> MSLRIDVDTNFPECVVDAGKVTLGTQQRQEMDPRLREKQNEIILRAVCALLNSGGGIIKAEIENKGYNYERHGVGLDVPPIFRSHLDKMQKENHFLIFVKSWNTEAGVPLATLCSNLYHRERTSTDVMDSQEALAFLKCRTQTPTNINVSNSLGPQAAQGSVQYEGNINVSAAALFDRKRLQYLEKLNLPESTHVEFVMFSTDVSHCVKDRLPKCVSAFANTEGGYVFFGVHDETCQVIGCEKEKIDLTSLRASIDGCIKKLPVHHFCTQRPEIKYVLNFLEVHDKGALRGYVCAIKVEKFCCAVFAKVPSSWQVKDNRVRQLPTREWTAWMMEADLEHHHHHH

The Schlafen family belongs to the interferon-stimulated genes and its members are involved in cell cycle regulation, T cell quiescence, inhibition of viral replication, DNA-repair and tRNA processing. Here, we present the cryo-EM structure of full-length human Schlafen 5 (SLFN5) and the high-resolution crystal structure of the highly conserved N-terminal core domain. SLFN5 binds tRNA as well as single- and double-stranded DNA, suggesting a potential role in transcriptional regulation. The N-terminal Slfn core domain (residues 1–336) is followed by a linker domain (residues 337–552) and a C-terminal helicase/ ATPase domain (residues 553–891).

To gain high resolution structural insights into human SLFN5, we crystallized the SLFN5 core domain (SLFN51–336). The core domain (38.9 kDa) behaves as a monomer in solution, as determined by right angle light scattering (RALS). SLFN51–336 crystallized in the space groups P3221 and P21, diffracting to 3.2 and 1.8 Å, respectively. The SLFN51- 336 structure depicts a horseshoe-like shape with a mixed α/β topology consisting of 10 α-helices and 14 β-sheets. The domain consists of an N-terminal and C-terminal lobe with respective bridging domain. Each lobe consists of four α-helices and five β-sheets and each bridging domain of one helix and two sheets. The SLFN51–336 structure comprises a zinc finger motif with the calculated anomalous map confirming the presence of a zinc ion. The zinc ion is coordinated by a histidine and three cysteine residues (H266, C268, C302, C303) that are highly conserved throughout the entire Schlafen protein family. The structure of SLFN51–336 shows similarity to the published structure of the N-terminal domain of rat Slfn13 (rSlfn1314–353).>[2x]RRATDTTPPTITVPSDIIAYRGEEFEF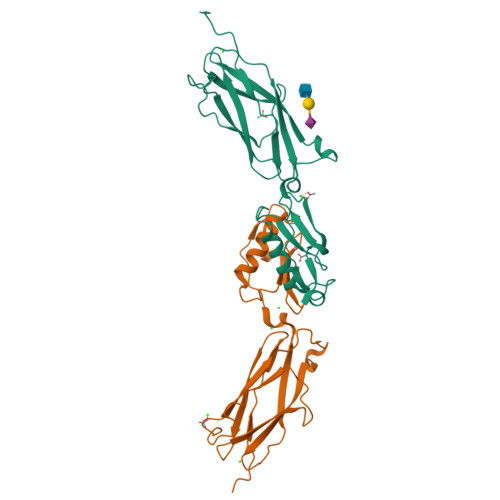YFEITDDSGQVKNIELSTFGKPLGLNWLEYSEDNFNVPGNATSDNPLRVRVHGTVPLNEPIPADKNRAQFTRTIRAWDAAGNVSSNITFVIKYRAQTDKYNPADPTITYVDRLSSLSPSEKNAVEAAVRAANPQIPAAARITVSANGTVTITYPDSSTDTITANRVVKDLASSR>SDPDPLQDFCVADLDGKAVSVNGHTCKPMSEAGDDFLFSSKLTKAGNTSTPNGSAVTELDVAEWPGTNTLGVSMNRVDFAPGGTNPPHIHPRATEIGMVMKGELLVGILGSLDSGNKLYSRVVRAGETFVIPRGLMHFQFNVGKTEAYMVVSFNSQNPGIVFVPLTLFG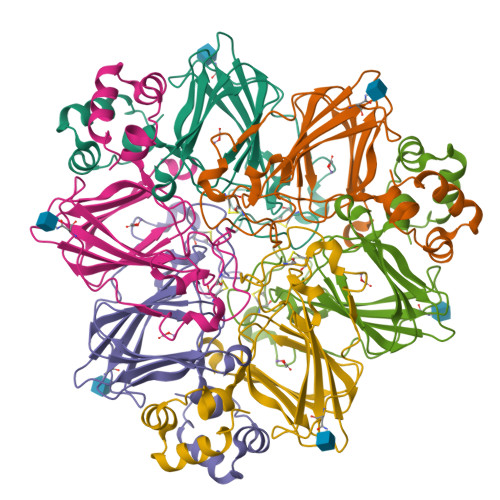SDPPIPTPVLTKALRVEAGVVELLKSKFAGGS[2x]>MISMKPRYKPDWESLREHTVPKWFDKAKFGIFIHWGIYSVPGWATPTGELGKVPMDAWFFQNPYAEWYENSLRIKESPTWEYHVKTYGENFEYEKFADLFTAEKWDPQEWADLFKKAGAKYVIPTTKHHDGFCLWGTKYTDFNSVKRGPKRDLVGDLAKAVREAGLRFGVYYSGGLDWRFTTEPIRYPEDLSYIRPNTYEYADYAYKQVMELVDLYLPDVLWNGMGWPEKGKEDLKYLFAYYYNKHPEGSVNDRWGVPHWDFKTAEYHVNYPGDLPGYKWEFTRGIGLSFGYNRNEGPEHMLSVEQLVYTLVDVVSKGGNLLLNVGPKGDGTIPDLQKERLLGLGEWLRKYGDAIYGTSVWERCCAKTEDGTEIRFTRKCNRIFVIFLGIPTGEKIVIEDLNLSAGTVRHFLTGERLSFKNVGKNLEITVPKKLLETDSITLVLE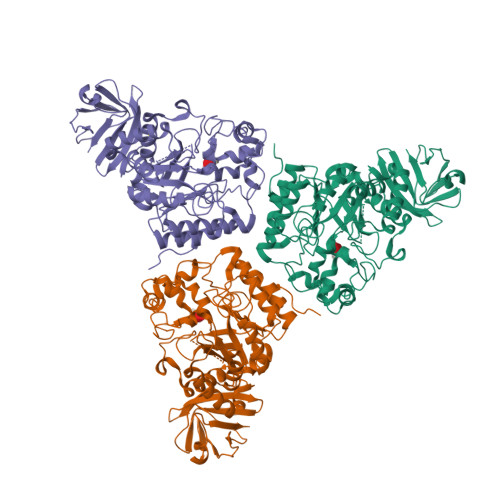AVEE[2x]>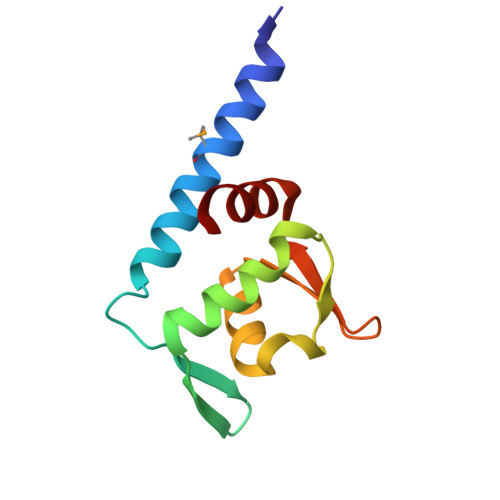 SNALKDVLNILLMDEISKLKDFLSNLDYIKPKVNIEEEIIEIRKEDIINALKLFKGKYEIEVDKIPKAVYVYLVKKNILFLYPQRGTLKPQSFLVWNAIKRVL> SGDEADRTLFVGNLETKVTEELLFELFHQAGPVIKVKIPKDKDGKPKQFAFVNFKHEVS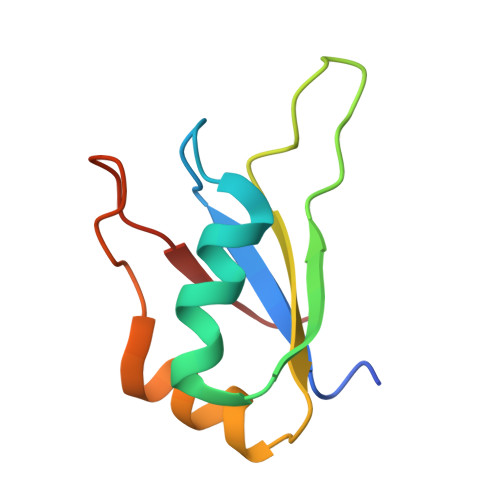VPYAMNLLNGIKLYGRPIKIQFRS>MATAQVTCVWDLKATLGEGPIWHGDTLWFVDIKQRKIHNYHPATGERFSFDAPDQVTFLAPIVGATGFVVGLKTGIHRFHPATGFSLLLEVEDAALNNRPNDATVDAQGRLWFGTMHDGEENNSGSLYRMDLTGVARMDRDICITNGPCVSPDGKTFYHTDTLEKTIYAFDL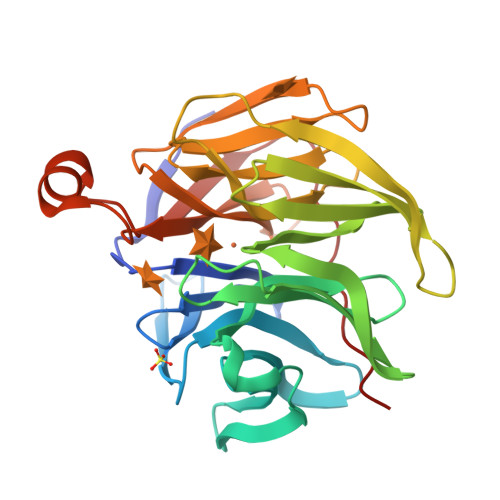AEDGLLSNKRVFVQFALGDDVYPDGSVVDSEGYLWTALWGGFGAVRFSPQGDAVTRIELPAPNVTKPCFGGPDLKTLYFTTARKGLSDETLAQYPLAGGVFAVPVDVAGQPQHEVRLV[2x]>GQDMVSPPPPIADEPLTVNTGIYLIECYSLDDKAQTFKVNAFLSLSWKDRRL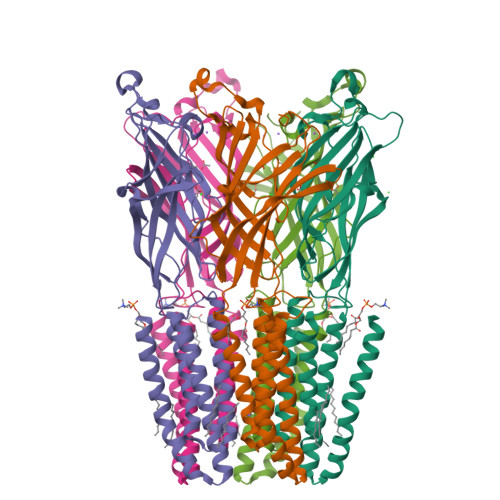AFDPVRSGVRVKTYEPEAIWIPEIRFVNVENARDADVVDISVSPDGTVQYLERFSARVLSPLDFRRYPFDSQTLHIYLIVRSVDTRNIVLAVDLEKVGKNDDVFLTGWDIESFTAVVKPANFALEDRLESKLDYQLRISRQYFSYIPNIILPMLFILFISWTAFWSTSYEANVTLVVSTLIAHIAFNILVETNLPKTPYMTYTGAIIFMIYLFYFVAVIEVTVQHYLKVESQPARAASITRASRIAFPVVFLLANIILAFLFFGF[5x]> MPQSKSRKIAILGYRSVGKSSLTIQFVEGQFVDSYDPTIENTFTKLITVNGQEYHLQLVDTA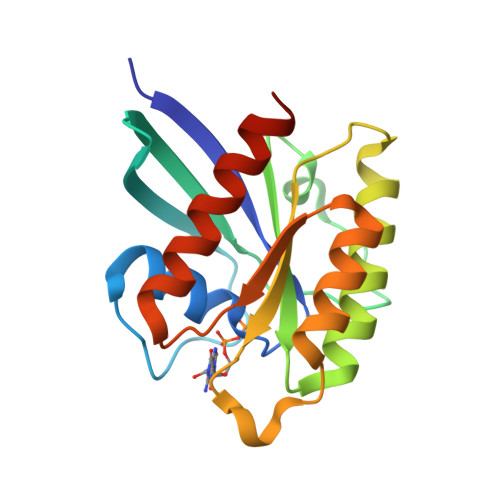GQDEYSIFPQTYSIDINGYILVYSVTSIKSFEVIKVIHGKLLDMVGKVQIPIMLVGNKKDLHMERVISYEEGKALAESWNAAFLESSAKENQTAVDVFRRIILEAEKLEHHHHHH>[5x]TKKSREEIVKEILGRANPNNIPIVDEQPVKVSFKYSLQDIYTADVGTDQVELGLWLVISWKDRSLSWSNECTTFNELTLPSKYIWLPHIEVYNSIGKPGIHSDQL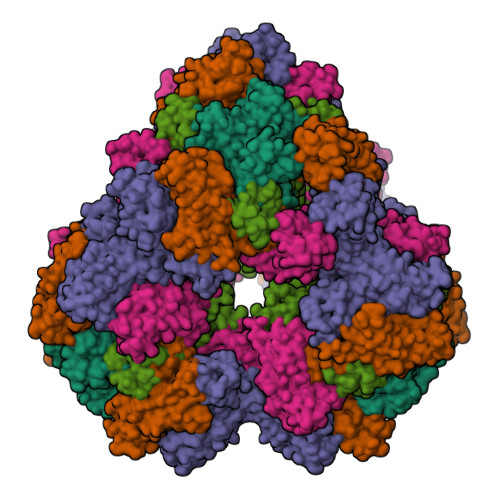VRVYKDGTVTFVPQYTIRFSCALENVTTEQGAACTLKFGPWTYDVRDLVLDESQQVDLTTYAGGERFQLIEAKQKVNKKTYPCCPQSFEDIELRVTFKKI> MVECITPEAIFIGANKQTQVSDIHKVKKIVAFGAGKTIALWDPIEPNNKGVYATLKGHEAEVTCVRFVPDSDFMVSASEDHHVKIWKFTDYSHLQCIQTIQHYSKTIVALSALPSLISVGCADGTISIWRQNIQNDEFGLAHEFTIKKGFFYPLCLSLSKVEEKKYLLAIGGTNVNVFIASFILSDSGIEKCRVVAELEGHEDWVKSLAFRHQETPGDYLLCSGSQDRYIRLWRIRINDLIDDSEEDSKKLTLLSNKQYKFQIDDELRVGINFEALIMGHDDWISSLQWHESRLQLLAATADTSLMVWEPDETSGIWVCSLRLGEMSSKGASTATGSSGGFWSCLWFTHERMDFFLTNGKTGSWRMWATKDNIICDQRLGISGATKDVTDIAWSPSGEYLLATSLDQTTRLFAPWIYDASGRKREIATWHEFSRPQIHGYDMICVETVTDTRFVSGGDEKILRSFDLPKGVAGMLQKFVGIQFEEKSEMPDSATVPVLGLSNKAGEDDANEDDEEEEGGNKETPDITDPLSLLECPPMEDQLQRHLLWPEVEKLYGHGFEITCLDISPDQKLIASACRSNNVQNAVIRIFSTENWLEIKPALPFHSLTITRLKFSKDGKFLLSVCRDRKWALWERNMEDNTFELRFKNEKPHTRIIWDADWAPLEFGNV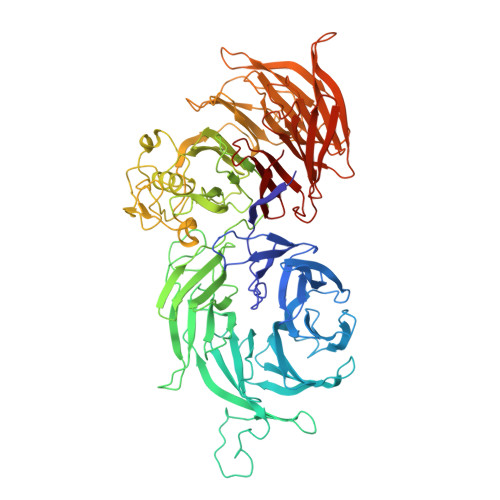FVTASRDKTVKVWRHQKEPADDYVLEASIKHTKAVTAISIHDSMIREKILISVGLENGEIYLYSYTLGKFELITQLNEDITPADKITRLRWSHLKRNGKLFLGVGSSDLSTRIYSLAYE> SPNSQYLKTRILDIYTPEQRAGIEKSEDWRQFSRRMDTHFPKLMNELDSVYGNNEALLPMLEMLLAQAWQSYSQRNSSLKDIDIARENNPDWILSNKQVGGVCYVDLFAGDLKGLKDKIPYFQELGLTYLYLMPLFKCPEGKSDGGYAVSSYRDVNPALGTIGDLREVIAALHEAGISAVVDFIFNHTSNEHEWAQRCAAGDPLFDNFYYIFPDRRMPDQYDRTLREIFPDQHPGGFSQLEDGRWVWTTFNSFQWDLNYSNPWVFRAMAGEMLFLANLGVDILRMDAVAFIWKQMGTSCENLPQAHALIRAFNAVMRIAAPAVFFKSQAIVHPDQVVQYIGQDECQIGYNPLQMALLWNTLATREVNLLHQALTYRHNLPEHTAW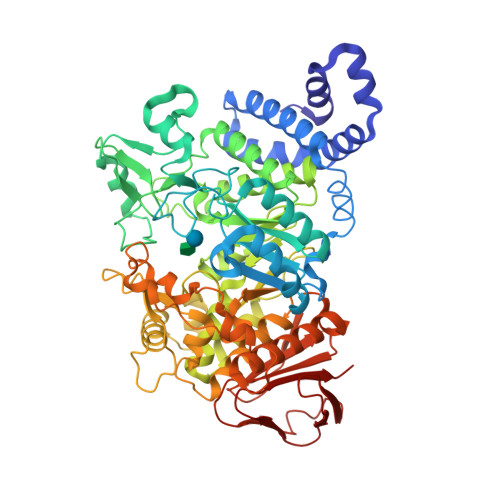VNYVRSHDDIGWTFADEDAAYLGISGYDHRQFLNRFFVNRFDGSFARGVPFQYNPSTGDCRVSGTAAALVGLAQDDPHAVDRIKLLYSIALSTGGLPLIYLGDEVGTLNDDDWSQDSNKSDDSRWAHRPRYNEALYAQRNDPSTAAGQIYQDLRHMIAVRQSNPRFDGGRLVTFNTNNKHIIGYIRNNALLAFGNFSEYPQTVTAHTLQAMPFKAHDLIGGKTVSLNQDLTLQPYQVMWLEIA The EDTA transporter system is composed of a periplasmic binding protein, EppA, and a type I ABC-type importer consisting of a heterodimer of its transmembrane domain components, EppB and EppC, and a dimer of its nucleotide binding domain component, EppD. EppA binds free EDTA, but not metal–EDTA complexes, restricting the ability of Chelativorans sp. BNC1 to use only weak metal–EDTA complexes that can dissociate to free EDTA, making it imperative to determine the biophysical mechanism of EppA’s binding specificity before any improvements to its binding capabilities can be engineered. Based on its three-domain, bilobate structure, the β2β1β3βnβ4 configuration of the core β-sheet of Domain III, and the two-β-strand hinge, EppA is a Class II Cluster C periplasmic binding protein. In summary, EppA’s affinity for EDTA, EDDA, and EGTA, and its putative affinity for other APC chelators via molecular docking, suggests that it is a general binding protein for aminopolycarboxylates.

Soaking the crystals with EDTA lowered their symmetry from P43212 to P212121, thereby doubling the molecules in the asymmetric unit to two; however, no EDTA molecules could be placed unambiguously into the orthorhombic structure after refining the model with EDTA in the ligand-binding cleft. Instead, two sulfate ions from the ammonium sulfate in the crystallization solution were present in the cleft of EppA. For both structures, all but the first four N-terminal residues (Gln27 through Leu30) of the mature protein (Gln27 through Glu563) were visible, and the C-terminal His-tag from pET30a(+) was visible through its first three His residues. Based on the relatively weak (e.g., no large, hydrophobic intermolecular interfaces) crystallographic and non-crystallographic protein–protein interactions in both the P43212 and P212121 crystal lattices, EppA is monomeric, which we confirmed by calculating a molecular mass of 63 kDa for the single chromatographic peak observed by analytical size-exclusion chromatography. Due to the high ammonium sulfate concentrations (1 to 2 M) in all of the conditions that EppA crystallized in, sulfate ions occupied EppA’s binding cleft, preventing formation of an EppA–EDTA complex. When 100 mM EDTA was added to the crystals, it caused the crystals to melt. To determine EppA’s EDTA-binding mechanism, we resorted to molecular docking.

>[2x]MNIRLHGLTTILSALVVLTAPTAVLAQDNLVTGELITTVNSGTPGKGGEVTFAVTRDITNWNVTSALGNNAVVRTVTLPIVPSAFMVQPDFTLKMNTDLLESAELTSTDPQTVVYRIREDAVWSDGVPITGDDFIYFWKTQNRRDCPECLINASYGHDFIETLEQDETGKVVTATFSEPFLGWQGLFMFLYPAHLAEKHGDIAESYNNFLSNEVPAWSGGPYMVESFDPGQLVTLVPNPKWYGEKGPYLDKLKFRIITDSTQQLTALENGEVDVIYPQGATQDMVEQAAGLDYLGIDFQMNPSANWYFMGLNSKAGPMSDIALRKAVLTAIDAGDLKAKTADPYLRNWPHMGSVMFLPNQAGYADRRGARGYGTGDVEKAKGILSEAGYKLSGGSLLDPSGKPVSTLRLSFPPGYPAANDMARLITGYIAPLGLKTDLLTGPNATADYLLSGNFDLHLNYFSQQVFPAVKAGQIFLRDTRQNYFGFNDPKIEEIIGKAAAASSIEESAAILSEADELAMDYAALFPIYQLPTALIYKEAILNLRDNPNQLGPAYNTAEWGLAELEHHHHHH> MQAAADRRTVEKTWKLMDKVVRLCQNPKLQLKNSPPYILDILPDTYQHLRLILSKYDDNQKLAQLSENEYFKIYIDSLMKKSKRAIRLFKEGKERMYEEQSQDRRNLTKLSLIFSHMLAEIKAIFPNGQFQGDNFRITKADAAEFWRKFFGDKTIVPWKVFRQCLHEV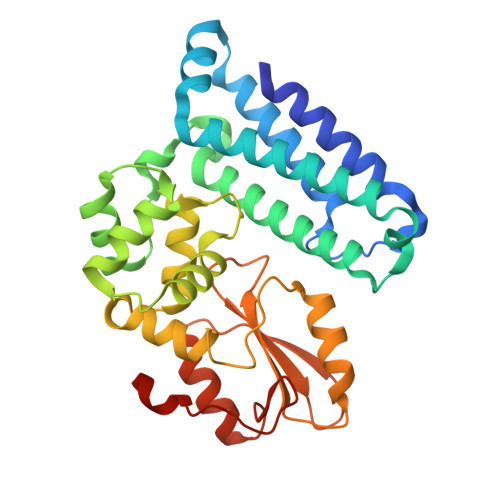HQISSGLEAMALKSTIDLTCNDYISVFEFDIFTRLFQPWGSILRNWNFLAVTHPGYMAFLTYDEVKARLQKYSTKPGSYIFRLSCTRLGQWAIGYVTGDGNILQTIPHNKPLFQALIDGSREGFYLYPDGRSYNPDLTGLAENLYFQ>[24x]MGCDAIQAAAALGEAGISSNEILELLAAAAELGLDPDAIQAAAQLGEAGISSEEIKELLRAAHELGLDPDAIAAAADLGQAGVSPVEILALLIAASVLGLDPDAIQAAAALGEAGISAEEIIELLTAARDLGLDPDAIQAAAQ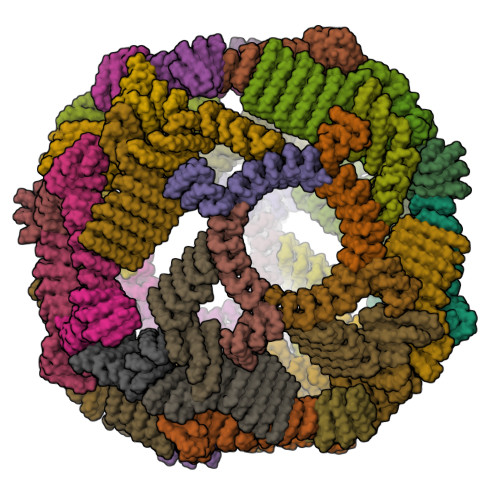LGEAGISSEEIKELLRAAHELGLDPDCIAAAADLGQAGISSSEITALLLAAAAIELAKRADDKDVREIVRDALELASRSTNDEVIRLALEAAVLAARSTDSDVLEIVKDALELAKQSTNEEVIKLALKAAVLAAKSTDEEVLEEVKEALRRAKESTDEEEIKEELRKAVEEAEGGSWLEHHHHHH;>[24x]MGDDLLLKLLELLVEQARVSAEFARRQGDEKMLEEVARKAEEVARKAEEIARKARKEGNLELALKALEILVRAAHVLAEIARERGNEELQKKAHKLAKEALRQVIEIAIRAIQEGNLELAIIALHISVRIAEVLLETRPDDREEIREQQAIFELLIAALEAAIRLEKLKEEGAPPEQIERVAEHGLERLKEIAKEISKEVDSPESKRIAYKIVAAAAEFLLKILAEGGATPEQLERVTEHALEVLKEVAKELADSPESVREAVRLISKLTQEGLKQLKEIGAPPEQIERVAEHGLEVLKEIAKYGSKLTDSPELKRELYRIISETAKELLKILAEGGATPEQLERVTKHALEVLKEVAKELADSPESGLAALAAIASLAKLGLEQLKEIGAPPEQQRRVTKAGIEAVREIYRYGRKLY>MPRGSRSRTSRMAPPASRAPQMRAAPRPAPVAQPPAAAPPSAVGSSAAAPRQPGLMAQMATTAAGVAVGSAVGHTLGHAITGGFSGGSNAEPARP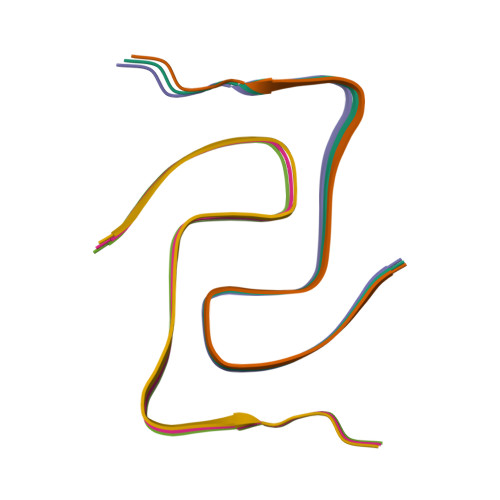DITYQEPQGTQPAQQQQPM[6x]>MAAAQPKYPAGATARRLARGCWSALWDYETPKVIVVRNRRLGVLYRAVQLLILLYFVWYVFIVQKSYQESETGPESSIITKVKGITTSEHKVWDVEEYVKPPEGGSVFSIITRVEATHSQTQGTCPESIRVHNATCLSDADCVAGELDMLGNGLRTGRCVPYYQGPSKTCEVFGWCPVEDGASVSQFLGTMAPNFTILIKNSIHYPKFHFSKGNIADRTDGYLKRCTFHEASDLYCPIFKLGFIVEKAGESFTELAHKGGVIGVIINWDCDLDLPASECNPKYSFRRLDPKHVPASSGYNFRFAKYYKINGTTTRTLIKAYGIRIDVIVHGQAGKFSLIPTIINLATALTSVGVGSFLCDWILLTFMNKNKVYSHKKFDKVCTPSHPSGSWPVTLARVLGQAPPEPGHRSEDQHPSPPSGQEGQQGAECGPAFPPLRPCPISAPSEQMVDTPASEPAQASTPTDPKGLAQL[3x]

The P2X2 receptor (P2X2R) is an adenosine triphosphate (ATP)-gated ion channel with few small-molecule modulators that exhibit poor pharmacological properties. It is known to be involved in the auditory system and has been proposed as a drug target for age- and noise-related hearing loss. Each P2X2 protomer is composed of intracellular N and C termini and two transmembrane (TM) helices (outer TM1 and pore-lining TM2) connected by a voluminous extracellular domain. Three P2X2 protomers intertwine to form the trimeric receptor, with each subunit adopting a dolphin-like shape, as first established for the zebrafish P2X4R (zfP2X4R).

To investigate the subtype-specific features of P2X2Rs, we used cryo-EM to determine the structure of full-length wild-type hP2X2R in an unliganded conformation. With a constricted pore and an absence of ATP in the orthosteric binding site, this structure represents an apo closed state —a key conformation for defining unliganded pockets and understanding the molecular changes resulting from subsequent agonist binding. We refined this cryo-EM reconstruction to 2.7 Å, allowing detailed structural visualization of this P2XR subtype. In the apo state conformation, the three TM2 helices are arranged in a “teepee” conformation to form the closed pore. In the apo closed state, the three symmetry-related side chains of I343 form the primary constriction gate (0.6 Å radius). In addition, another constriction formed by the symmetry-related side chains of T350 comprises a second, more cytoplasmic gate (1.1 Å radius). The primary constriction gate in the apo closed state is only 3.7 Å deep into the plasma membrane, as measured from the start of TM2 (Cα of L338 to Cα of I343), and thus the TMD forms a teepee shape. In addition, the surface-accessible volume of the orthosteric binding pocket in the hP2X2R is ~2,700 ± 400 Å3 as calculated by the program Fpocket, similar to that of the hP2X4R (~2,700 ± 19 Å3) and the rP2X7R (~2,700 ± 35 Å3), but strikingly smaller than the binding pocket volumes of the hP2X1R (~3,300 ± 200 Å3) and the hP2X3R (~5,100 ± 20 Å3). In agreement with these predictions, we observed V60 at the extracellular end of TM1 interacting with I339 of the neighboring protomer, D273 on a β-turn in the lower body at an interface with the TMD, and G353 on TM2, directly next to one of the pore-lining residues V354. The simulations using our apo closed state structure reveal that the left flipper is a conformationally flexible region, with an average fluctuation of 2.78 ± 0.81 Å calculated as RMS fluctuation (RMSF) across the three chains and all replicates.Clathrin mediates vesicular transport between post‐Golgi membranes in eukaryotes and is targeted to specific membranes by interactions with clathrin adaptor proteins. A total of 3 consensus clathrin‐binding peptide sequences have been identified and structural studies show that each binds distinct sites on the clathrin heavy chain N‐terminal domain (NTD). We have solved high‐resolution structures of NTD bound to peptide motifs from the cellular clathrin adaptors β2 adaptin and amphiphysin plus a putative viral clathrin adaptor, hepatitis D virus large antigen (HDAg‐L). Surprisingly, with each peptide we observe simultaneous peptide binding at multiple sites on NTD and viral peptides binding to the same sites as cellular peptides.

The viral peptides (HDAg‐L1pep and HDAg‐L2pep) bound at a similar site on NTD. However, in both cases only 2 consecutive hydrophobic side chains could be observed in the hydrophobic pocket (“IL” and “LL” in the cases of HDAg‐L1pep and HDAg‐L2pep, respectively). Interestingly, for both HDAg‐L1pep and HDAg‐L2pep the residues bound at the clathrin box do not match predictions based on alignments to the CBM consensus sequence, 18: in HDAg‐L1pep residues “ILFPA” occupy the positions corresponding to the LΦxΦ[DE], whereas in HDAg‐L2pep the residues “LLES”, including a C‐terminal serine residue that is non‐native and was added to the peptide to aid solubility, occupy the positions equivalent to the first 4 residues of the LΦxΦ[DE] consensus. The HDAg‐L2pep peptide could also be observed binding at the arrestin site, although the interaction was less extensive. The binding was largely similar to that observed for the cellular CBM peptides: the side chains of the 2 consecutive leucine residues bound at the hydrophobic cleft and their backbone atoms interacted with the side chain of Q192. In addition to binding at the clathrin and arrestin boxes, in 3 of the NTD:peptide co‐crystal structures solved (Amph4T1pep, HDAg‐L1pep and HDAg‐L2pep) a bound peptide could be observed lying across the interface between blades 6 and 7 of the NTD β‐propeller. In the co‐structure with Amph4T1pep a phenylalanine side chain projects deep into this pocket while in the HDAg‐L1pep and HDAg‐L2pep structures the side chains of a leucine residue and proline residue, respectively, bind less deeply. In all structures a hydrophobic side chain (leucine in Amph4T1pep and HDAg‐L2pep, isoleucine in HDAg‐L1pep) covers a surface hydrophobic patch formed by the hydrophobic portion of the R297 side chain and the hydrophobic faces of the peptide bonds between NTD residues 298‐300 on the surface of β‐propeller blade 6, and in all structures the backbone carbonyl oxygen of R297 forms a hydrogen bond with a backbone amide nitrogen of the bound peptide. Despite the similar molecular interactions made between the Royle box and the bound peptides, we note that the direction of the peptide chain differs between HDAg‐L1pep and Amph4T1pep/HDAg‐L2pep.

>[2x]GSMAQILPIRFQEHLQLQNLGINPANIGFSTLTMESDKFICIREKVGEQAQVVIIDMNDPSNPIRRPISADSAIMNPASKVIALKAGKTLQIFNIEMKSKMKAHTMTDDVTFWKWISLNTVALVTDNAVYHWSMEGESQPVKMFDRHSSLAGCQIINYRTDAKQKWLLLTGISAQQNRVVGAMQLYSVDRKVSQPIEGHAASFAQFKMEGNAEESTLFCFAVRGQAGGKLHIIEVGTPPTGNQPFPKKAVDVFFPPEAQNDFPVAMQISEKHDVVFLITKYGYIHLYDLETGTCIYMNRISGETIFVTAPHEATAGIIGVNRKGQVLSVCVEEENIIPYITNVLQNPDLALRMAVRNNLAGAEEL;>SPRLPLLES[6x]> GADAAVIEKLEAGFKKLEAATDCKSLLKKYLTKEVFDKLKDKKTSLGATLLDVIQSGVENLDSGVGIYAPDAEAYTLFAPLFDPIIEDYHVGFKQTDKHPNKDFGDVNSFVNVDPEGKFVISTRVRCGRSMQGYPFNPMLTESQYKEMEAKVSSTLSSLEGELKGTYYPLTGMSKEVQQKLIDDHFLFKEGDRFLQAANAMRYWPAGRGIYHNDNKTFLVWVNEEDHLRIISMQMGGDLGQVFRRLTSAVNEIEKRIPFSHHDRLGFLTFCPTNLGTTVRASVHIILPKLAANRAKLEEVAGKYNLQVAGTRGEHTEAEGGIYDISNKRRMGLTEFQA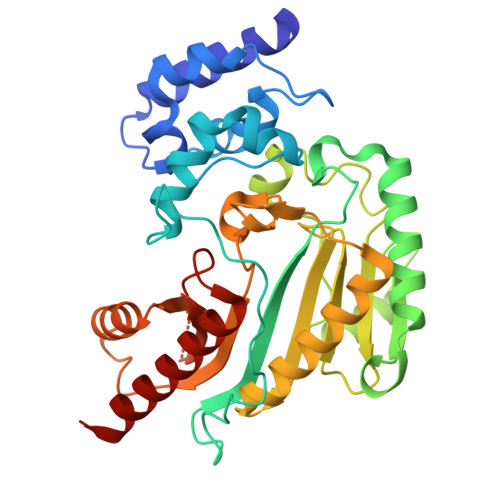VKEMQDGILELIKIEKEM Various transport systems are present to maintain intracellular Cu homeostasis, including the prokaryotic plasmid‐encoded multiprotein pco operon, which is generally assigned as a defense mechanism against elevated Cu concentrations. 23 While PcoA is a periplasmic multicopper oxidase, distantly related to CueO, PcoB resides in the outer membrane and has an elusive function. Here we structurally and functionally characterize the outer membrane component of the Pco system, PcoB, recovering a 2.0 Å structure, revealing a classical β‐barrel architecture. Aggregated, our findings indicate that PcoB serves to permit Cu import.

In contrast, N‐terminally truncated PcoB, PcoBΔ27−81, a form that does not alter the Cu‐binding properties, successfully yielded crystals in the presence of the detergent C8E4, which diffracted to 2.0 Å. Instead, the structure was determined using single‐wavelength anomalous diffraction (SAD) based on SeMet‐data and refined to R/Rfree = 0.22/0.26. The structure discloses a classical β‐barrel, formed by 12 antiparallel strands that span the outer membrane in vivo. However, the architecture of the PcoB barrel is flattened as a consequence of intra‐barrel contacts between charged amino acids, thus restricting the width, whereas these interactions of OmpLA are caused by hydrophobicity. Strikingly, a 12 × 18 Å wide cavity is present on the extracellular side (top right), as established by condensed loops between strands in the region leaving the aperture uncovered. From this region, a funnel‐like pore is penetrating almost the entire barrel, becoming narrower towards the periplasm, with a remarkably electronegative funnel surface throughout (bottom right). Along the pore, multiple negatively charged‐paired residues are present, in particular: E130‐E223 towards the extracellular side, D97‐E207 and N115‐Q179 towards the periplasm, which are both placed perpendicular to E187. The E130‐E223 and D97‐E207 pairs are both highly conserved among PcoB proteins, and form interacting carboxylic acid‐carboxylate hydrogen bonds that assist in flattening the barrel, and at the same time lines the pore. However, the structure was obtained in Cu‐free conditions, and consequently there are no indications of the metal in the pore. In contrast to the extracellular side, the waterline of the pore becomes partially obstructed at the intersection between D97, E187, D209 and E207, with D209 and the adjacent Y184, being in proximity to the periplasm and yet capping the pathway together with L183.

> GHAIHDSAINYLVLLDQLEWQRSDNTNNFSWSVNSWIGGDTDRIWLKSEGERSNGETEAAEAQLLWGHAVGPWWDLVAGVRQDFRPASARTWAAVGFQGLALYNFESEITGFVSNGGKAALRLGGEYDVLLTNRLILQPSYEVNFYSQDDESRGRGRGLTDTELGLRLRYEIRREFAPYIGVSWNQLYGKTSDMAKREGEKDHQVVFLAGARIWF>ADKELKFLVVDDESTMRRIVRNLLKELGFNNVEEAEDGVDALNKLQAGGYGFVISDWMMPNMDGLELLKTIRADGAMSALPVLMVTARAKKENIIAAAQAGASGYVVKPFTAATLEEKLNKIF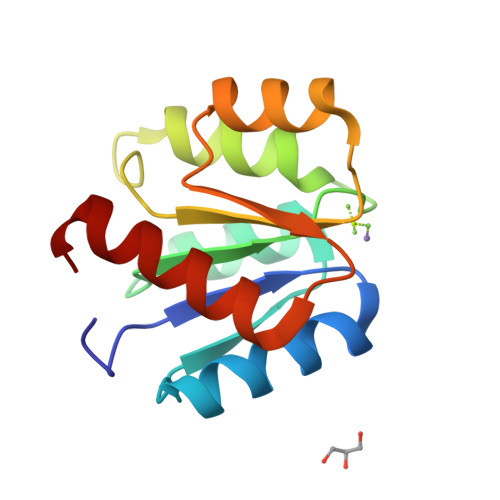EKLGM[2x]> SSLDDKPQFPGASAEFIDKLEFIQPNVISGIPIYRVMDRQGQIINPSEDPHLPKEKVLKLYKSMTLLNTMDRILYESQRQGRISFYMTNYGEEGTHVGSAAALDNTDLVFGQYREAGVLMYRDYPLELFMAQCYGNISDLGKGRQMPVHYGCKERHFVTISSPLATQIPQAVGAAYAAKRANANRVVICYFGEGAASE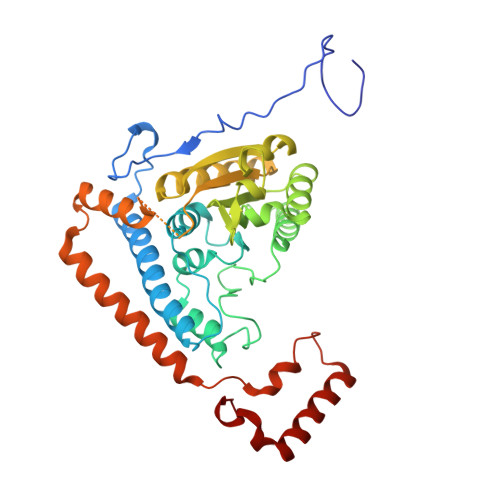GDAHAGFNFAATLECPIIFFCRNNGYAISTPTSEQYRGDGIAARGPGYGIMSIRVDGNDVFAVYNATKEARRRAVAENQPFLIEAMTYAIGHASTSDDSSAYRSVDEVNYWDKQDHPISRLRHYLLSQGWWDEEQEKAWRKQSRRKVMEAFEQAERKPKPNPNLLFSDVYQEMPAQLRKQQESLARHLQTYGEHYPLDHFDK> MEIPVIEPLFTKVTEDIPGAEGPVFDKNGDFYIVAPEVEVNGKPAGEILRIDLKTGKKTVICKPEVNGYGGIPAGCQCDRDANQLFVADMRLGLLVVQTDGTFEEIAKKDSEGRRMQGCNDCAFDYEGNLWITAPAGEVAPADYTRSMQEKFGSIYCFTTDGQMIQVDTAFQFPDGIAVRHMNDGRPYQLIVAETPTKKLWSYDIKGPAKIENKKVWGHIPGTHEGGANGMDFDEDNNLLVANWGSSHIEVFGPDGGQPKMRIRCPFEKPSNLHFKPQTKTIFV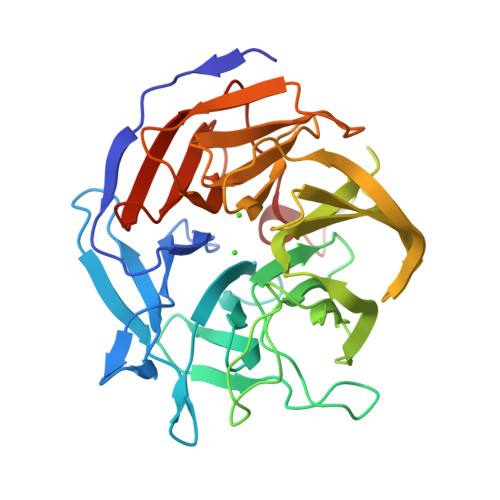TEHENNAVWKFEWQRNGKKQYCETLKFGIF1,1,1-tris(fluoranyl)propan-2-one | C3 H3 F3 O 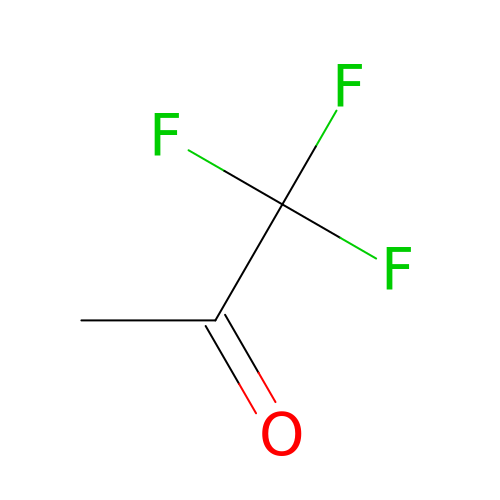| FHUDAMLDXFJHJE-UHFFFAOYSA-N>[2x]MDKENK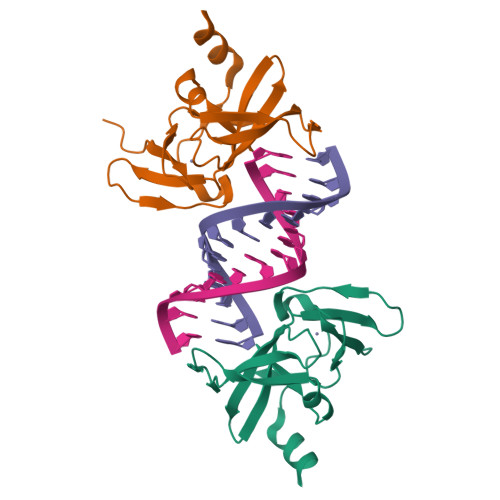KLLCRKCKALACYTADVRVIEESHYTVLGDAFKECFVSRPHPKPKQFSSFEKRAKIFCARQNCSHDWGIHVKYKTFEIPVIKIESFVVEDIATGVQTLYSKWKDFHFEKIPFDPAEMSKLEH> G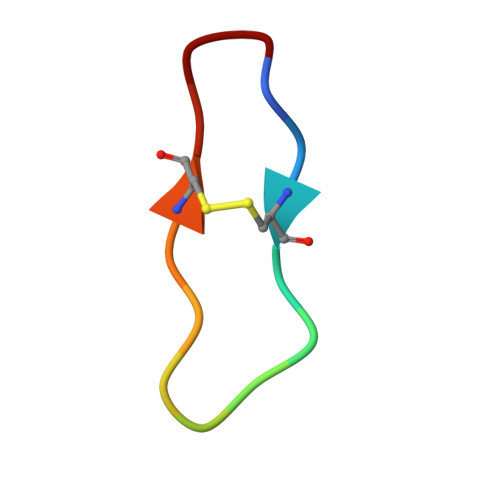RCTKSIPPICFPD6-(3-oxidanylpropyl)-2-(1,3,6-trimethyl-2-oxidanylidene-benzimidazol-5-yl)benzo[de]isoquinoline-1,3-dione | C25 H23 N3 O4 | 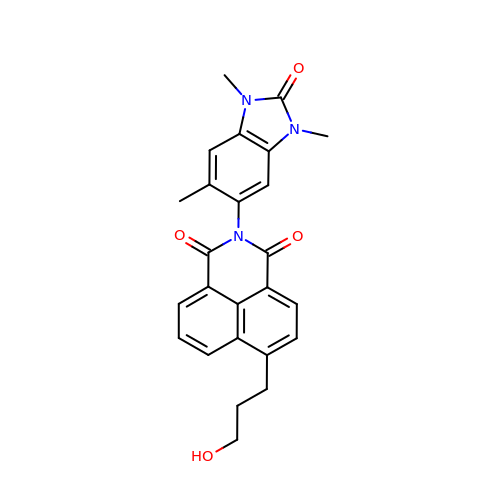OFWWWKWUCDUISA-UHFFFAOYSA-N Ribonucleotide reductase (RNR) is a key enzyme in all domains of life, utilizing radical chemistry for the synthesis of deoxyribonucleotides by substitution of the 2′ OH-group of a ribose 5′phosphate with a hydrogen. The strictly aerobic class I RNRs are comprised of two homodimeric subunits: a large catalytic subunit R1, where ribonucleotide reduction takes place, and a small radical-generating subunit R2. R2a proteins utilize an oxygen-activated di-ferrous metal site to generate a stable FeIII/FeIII-tyrosyl radical (Y·) cofactor, whereas R2b proteins generate a MnIII/MnIII-Y·. R2c proteins generate a MnIV/FeIII cofactor and the recently discovered class R2d—a MnIV/MnIII cofactor. These dimetal centers reside in a ferritin-like scaffold, and are coordinated by two histidine residues and four carboxylate ligands.

In addition, we have introduced an R2lox-like L61G mutation in the second coordination sphere in close proximity to the N-terminal metal binding site (site 1) and investigated its effect on the structure and protein metallation. The structure of the metal-free L61G variant closely resembles the WT BaR2b. The structure of the putative superoxide passage to the metal in site 2 was not affected by the mutation. The substitution of Leu61 with Gly allows the Phe165 side chain, located on αE, to adopt an alternative conformation, occupying the vacant space, creating a larger hydrophobic cavity around the metal center. Interestingly, the distorted part of the αE (residue stretch 159–168), adopting a π/310-helical conformation in all L61G structures, has an increased B-factor for the Cα atoms, suggesting that the mutation has a destabilizing effect in this region. Additionally, the mutation renders a larger surface-connected cavity between helices αB (residues 46–76) and αD (residues 125–140), gated by Met1 and Glu127. Overall, in all structures reported in this study, the first 288 residues could be traced in the electron density, leaving the last 34 C-terminal residues disordered. The electron density is well-defined, except for a flexible poly-glutamate loop region E275–E278.

>[2x]MRAVNWNKKEDDFSLMFWKQNIAQFWTEEEIAVSSDKNTWVQLSKEEQIAYKRVLGGLTLGDTKQGGEGMPLVLVHLENLQAKSVLAFMGAMEEVHAKSYSHIFTTLATEEEIDEIFDWVDTHPLLEKKAGIITSYYRRLLKPEVTKKELYMAMVASVFLESYLFYSGFFYPLYLAGQGKLTASGEIINLIIRDESIHGVFVGILAQQIFAELSAEDQQEVQKETQELLMELYEIEMAYTEEIYTSIGLVEDVNRFVRYNANKGLMNLGLEPKFEEEEINPIVLNGLRTDTKNHDFFSVKGNGYVKATNVEKLSDDDFVFNF>[2x]APDW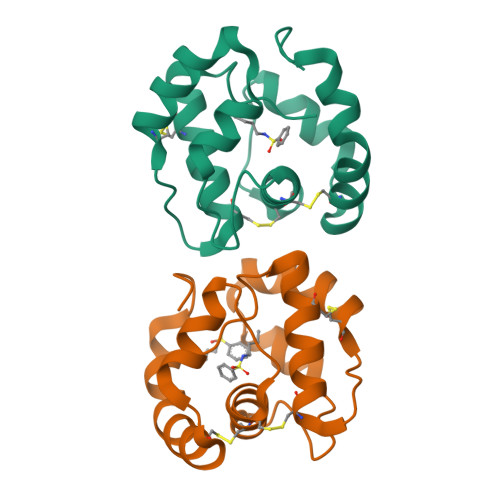VPPEVFDLVAEDKARCMSEHGTTQAQIDDVAKGNLVNEPSITCYMYCLLEAFSLVDDEANVDEDIMLGLLPDQLQERAQSVMGKCLPTSGSDNCNKIYNLAKCVQESAPDVWFVI>MEGTGVVAVYGNGAITEAKK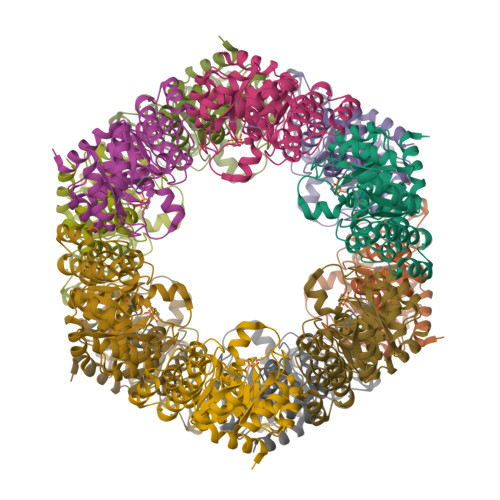SPFSVKVGLAQMLRGGVIMDVVNAEQARIAEEAGACAVMALERVPADIRAQGGVARMSDPQMIKEIKQAVTIPVMAKARIGHFVEAQILEAIGIDYIDESEVLTLADEDHHINKHNFRIPFVCGCRNLGEALRRIREGAAMIRTRGEAGTGNIIEAVRHVRSVNGDIRVLRNMDDDEVFTFAKKLAAPYDLVMQTKQLGRLPVVQFAAGGVATPADAALMMQLGCDGVFVGSGIFKSGDPARRARAIVQAVTHYSDPEMLVEVSCGLGEAM[4x]> MSTSTSQIAVEYPIPVYRFIVSVGDEKIPFNSVSGLDISYDTIEYRDGVGNWFKMPGQSQSTNITLRKGVFPGKTELFDWINSIQLNQVEKKDITISL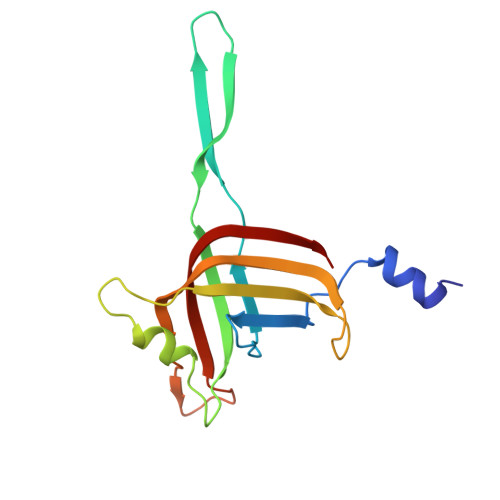TNDAGTELLMTWNVSNAFPTSLTSPSFDATSNDIAVQEITLMADRVIMQAV>MQRLFLLVAVMLLSGCLTAPPKEAARPTLMPRAQSYKDLTHLPAPTGKIFVSVYNIQDETGQFKPYPASNFSTAVPQSATAMLVTALKDSRWFIPLERQGLQNLLNERKIIRAAQENGTVAINNRIPLQSLTAANIMVEGSIIGYESNVKSGGVGARYFGIGADTQYQLDQIAVNLRVVNVSTGEILSSVNTSKTILSYEVQAGVFRFIDYQRLLEGEV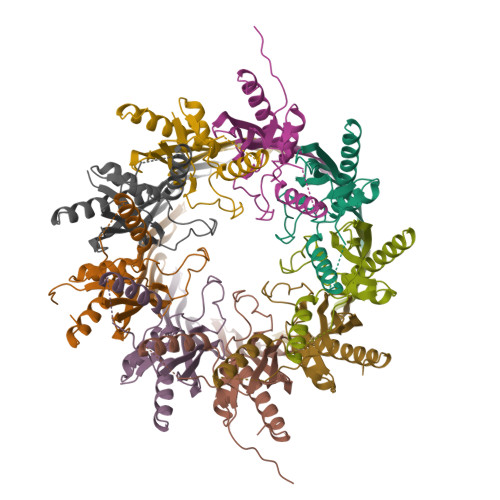GYTSNEPVMLCLMSAIETGVIFLINDGIDRGLWDLQNKAERQNDILVKYRHMSVPPES[9x]>[2x]GSHMASNDLIYQDEHASLQPLEGRTVAVIGYGIQGRAFAANLRDSGVAVRVGNIDDRYFELARAEGHRVTNIAEAVAHADIVLLLIPDEAHGAVFDVDIAPNLRDGALLCVAH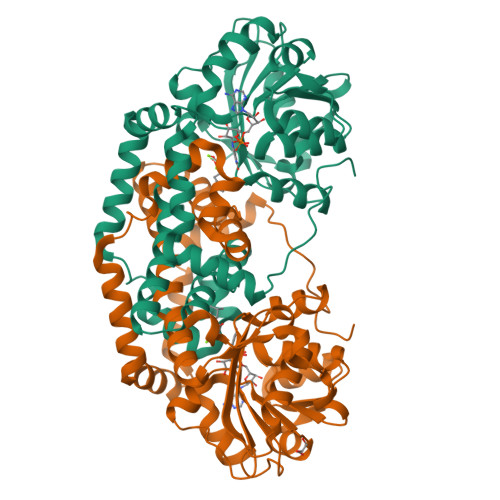GHSLVQGDVRPLPGRDLAMLAPRMYGDPIRRYYLAGQGAPAYFDIVADHTGRARDRVLAIARAVGFTRAGVMALGYRQETFLDLFQEQFLAPALVDLVETGFQVLVERGFNPKAALLEVYGSGQMGKMMLDGADIGLDEVVALQGSPTCQVGYHRWRGRTLPTAVRELAARVLDQIEGGDFSAYLKEQASNDYASLDDARRAALKRPLNVAHAQVRAAFRFPTEAAGGLYQAAQAPADVEPEAAR> KKISQYACQRRTTLNNYNQLFTDALDI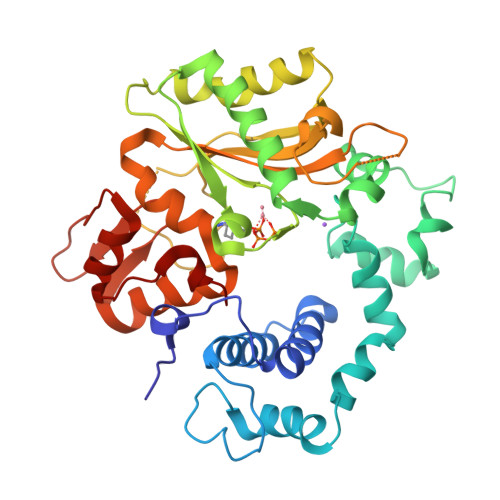LAENDELRENEGSCLAFMRASSVLKSLPFPITSMKDTEGIPCLGDKVKSIIEGIIEDGESSEAKAVLNDERYKSFKLFTSVFGVGLKTAEKWFRMGFRTLSKIQSDKSLRFTQMQKAGFLYYEDLVSCVNRPEAEAVSMLVKEAVVTFLPDALVTMTGGFRRGKMTGHDVDFLITSPEATEDEEQQLLHKVTDFWKQQGLLLYCDILESTFEKFKQPSRKVDALDHFQKCFLILKLDHGRVHSEKSGQQEGKGWKAIRVDLVMCPYDRRAFALLGWTGSRQFERDLRRYATHERKMMLDNHALYDRTKRVFLEAESEEEIFAHLGLDYIEPWERNA During infection of mammalian hosts, African trypanosomes thwart immunity using antigenic variation of the dense Variant Surface Glycoprotein (VSG) coat, accessing a large repertoire of several thousand genes and pseudogenes, and switching to antigenically distinct copies. In the salivary glands of the fly, the pathogen adopts the metacyclic form and expresses a limited repertoire of VSG genes specific to that developmental stage. We present here three novel metacyclic form VSG N-terminal domain crystal structures (mVSG397, mVSG531, and mVSG1954) and show that they mirror closely in architecture, oligomerization, and surface diversity the known classes of bloodstream form VSGs. The VSG protein can be roughly divided into three functional units: the signal peptide for delivery to the cell surface (and which is cleaved during translocation), a large N-terminal domain (NTD) that forms the bulk of the molecule, and the smaller C-terminal domain (CTD) that is tethered to the NTD by a flexible linker that can often be removed by endogenous and exogenous proteases.

VSGs 397 and 531 fall within Class A by homology analysis, whereas VSG1954 is a member of Class B. More specifically, by using the classification system outlined in Cross et al., mVSG397 belongs to Class A1 (similar to VSG522, which shares 72% sequence identity with Trypanosoma brucei rhodesiense VSGsur (GenBank: ATI14856), whose unusual structure was recently determined), mVSG531 to Class A2 (the same as VSG1 and VSG2), and VSG1954 to Class B. The conservation extends to the location of the four cysteine disulfides bridges concentrated at the top-lobe of the monomer. As with VSG3, and in contrast to Class A VSGs, mVSG1954 behaves as a monomer in solution and crystallized as a monomer in the asymmetric unit of the crystal. The ability of mVSG1954 to exist as a monomer is further corroborated by SEC-MALS analysis (size exclusion chromatography coupled to multi-angle light scatting). Also, like VSG3, while a monomer in the asymmetric unit, the mVSG1954 NTD exists as a crystallographic trimer that is highly similar to that of VSG3. Altogether, these data argue that, diverging from the dimers of Class A VSGs, members of Class B may adopt a trimeric oligomeric state, at least in solution and crystals, and possibly on the membrane. In contrast to the structure of VSG3, the NTD of mVSG1954 does not show any evidence in the crystals of O-linked glycosylation, despite possessing a close consensus sequence to the motif shown previously to often contain this PTM. Using intact protein mass spectrometry, the absence of such a sugar on the conserved loop at S321 was confirmed (the residue predicted to be glycosylated from the consensus sequence), although a hexose residue was found on the full length protein, even after PNGase treatment. This additional hexose may be located on the highly glycosylated CTD or on a novel site in the NTD that was, nonetheless, not seen to be glycosylated in the crystals.

> ADVAAGSNAESYAVLCTLVQLTKATKPSVPKSKIIDEVYNVAAAIGLAIRGDAVVKNCIDKKDSKYSDLTDSDIAKKAYTERTWPVAQAGAAKLASSGEKEKYASWTHRKYTEKQKLKVHVLTAAISDVKQRADKLNKPDKLAELTGALSNSLYGNGKSNADTATLPAGGSHISMCGPADGTQGGSIVGKALKFDLICLCGKQSADSGTGEKACHEFSPLPATAIAENAAINADWATIEQGCKTVAGAPSLTPESIHAALQAFYRHAGVPKGNTRNRYTTVGAPAGSGATGCDGIGGSNGGKCAAYNKAQFEAGTGPYWATQMKAAAETLVELRGQEQKLAALEAEALALNSTLDGMQHD> HHHHHHDDTS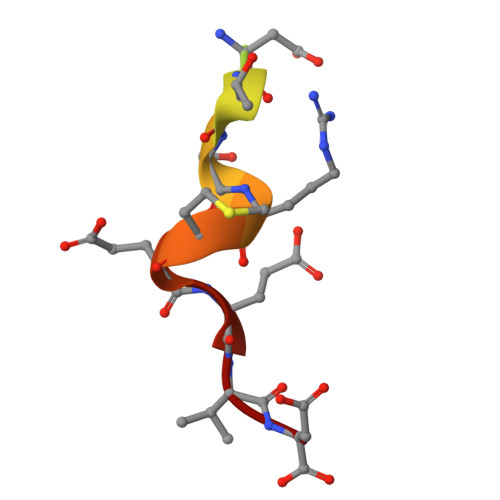RMEEVD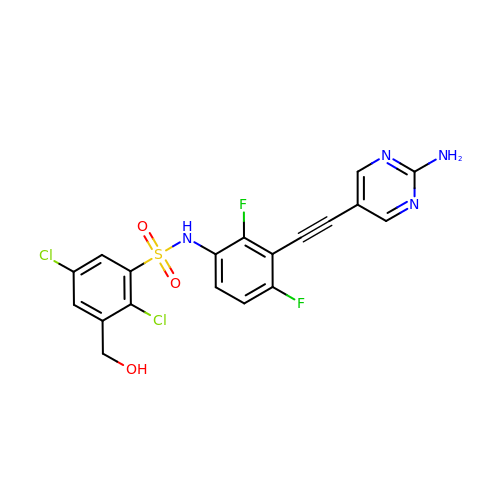N-{3-[(2-aminopyrimidin-5-yl)ethynyl]-2,4-difluorophenyl}-2,5-dichloro-3-(hydroxymethyl)benzene-1-sulfonamide | C19 H12 Cl2 F2 N4 O3 S | VJXAWOQPYMAEFQ-UHFFFAOYSA-N2-(4-phenoxyphenoxy)-5-[(3R)-1-(prop-2-enoyl)piperidin-3-yl]pyridine-3-carboxamide | C26 H27 N3 O4 | 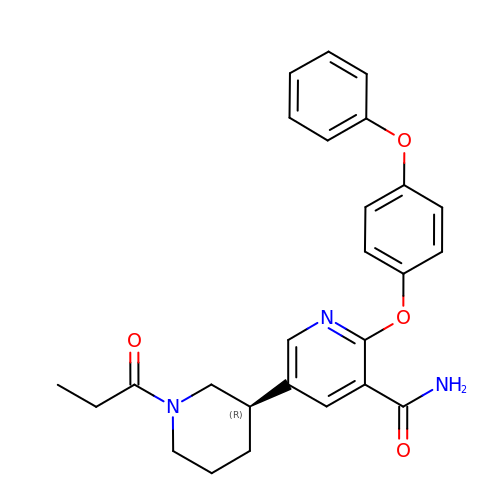KPAVXBRYORHPKS-SFHVURJKSA-N> MFLYNLTLQRATGISFAIHGNFSGTKQQEIVVSRGKILELLRPDPNTGKVHTLLTVEVFGVIRSLMAFRLTGGTKDYIVVGSDSGRIVILEYQPSKNMFEKIHQETFGKSGCRRIVPGQFLAVDPKGRAVMISAIEKQKLVYILNRDAAARLTISSPLEAHKANTLVYHVVGVDVGFENPMFACLEMDYEEADNDPTGEAAANTQQTLTFYELDLGLNHVVRKYSEPLEEHGNFLITVPGGSDGPSGVLICSENYITYKNFGDQPDIRCPIPRRRNDLDDPERGMIFVCSATHKTKSMFFFLAQTEQGDIFKITLETDEDMVTEIRLKYFDTVPVAAAMCVLKTGFLFVASEFGNHYLYQIAHLGDDDEEPEFSSAMPLEEGDTFFFQPRPLKNLVLVDELDSLSPILFCQIADLANEDTPQLYVACGRGPRSSLRVLRHGLEVSEMAVSELPGNPNAVWTVRRHIEDEFDAYIIVSFVNATLVLSIGETVEEVTDSGFLGTTPTLSCSLLGDDALVQVYPDGIRHIRADKRVNEWKTPGKKTIVKCAVNQRQVVIALTGGELVYFEMDPSGQLNEYTERKEMSADVVCMSLANVPPGEQRSRFLAVGLVDNTVRIISLDPSDCLQPLSMQALPAQPESLCIVEMGGTEKQDELGERGSIGFLYLNIGLQNGVLLRTVLDPVTGDLSDTRTRYLGSRPVKLFRVRMQGQEAVLAMSSRSWLSYSYQSRFHLTPLSYETLEFASGFASEQCPEGIVAISTNTLRILALEKLGAVFNQVAFPLQYTPRKFVIHPESNNLIIIETDHNAYTEATKAQRKQQMAEEMVEAAGEDERELAAEMAAAFLNENLPESIFGAPKAGNGQWASVIRVMNPIQGNTLDLVQLEQNEAAFSVAVCRFSNTGEDWYVLVGVAKDLILNPRSVAGGFVYTYKLVNNGEKLEFLHK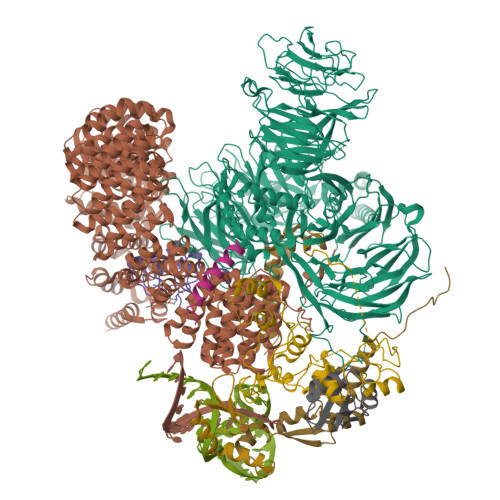TPVEEVPAAIAPFQGRVLIGVGKLLRVYDLGKKKLLRKCENKHIANYISGIQTIGHRVIVSDVQESFIWVRYKRNENQLIIFADDTYPRWVTTASLLDYDTVAGADKFGNICVVRLPPNTNDEVDEDPTGNKALWDRGLLNGASQKAEVIMNYHVGETVLSLQKTTLIPGGSESLVYTTLSGGIGILVPFTSHEDHDFFQHVEMHLRSEHPPLCGRDHLSFRSYYFPVKNVIDGDLCEQFNSMEPNKQKNVSEELDRTPPEVSKKLEDIRTRYAF;> MTDRYTIHSQLEHLQSKYIGTGHADTTKWEWLVNQHRDSYCSYMGHFDLLNYFAIAENESKARVRFNLMEKMLQPCGPPADKPEEN;> MAKIAKTHEDIEAQIREIQGKKAALDEAQGVGLDSTGYYDQEIYGGSDSRFAGYVTSIAATELEDDDDDYSSSTSLLGQKKPGYHAPVALLNDIPQSTEQYDPFAEHRPPKIADREDEYKKHRRTMIISPERLDPFADGGKTPDPKMNARTYMDVMREQHLTKEEREIRQQLAEKAKAGELKVVNGAAASQPPSKRKRRWDQTADQTPGATPKKLSSWDQAETPGHTPSLRWDETPGRAKGSETPGATPGSKIWDPTPSHTPAGAATPGRGDTPGHATPGHGGATSSARKNRWDETPKTERDTPGHGSGWAETPRTDRGGDSIGETPTPGASKRKSRWDETPASQMGGSTPVLTPGKTPIGTPAMNMATPTPGHIMSMTPEQLQAWRWEREIDERNRPLSDEELDAMFPEGYKVLPPPAGYVPIRTPARKLTATPTPLGGMTGFHMQTEDRTMKSVNDQPSGNLPFLKPDDIQYFDKLLVDVDESTLSPEEQKERKIMKLLLKIKNGTPPMRKAALRQITDKAREFGAGPLFNQILPLLMSPTLEDQERHLLVKVIDRILYKLDDLVRPYVHKILVVIEPLLIDEDYYARVEGREIISNLAKAAGLATMISTMRPDIDNMDEYVRNTTARAFAVVASALGIPSLLPFLKAVCKSKKSWQARHTGIKIVQQIAILMGCAILPHLRSLVEIIEHGLVDEQQKVRTISALAIAALAEAATPYGIESFDSVLKPLWKGIRQHRGKGLAAFLKAIGYLIPLMDAEYANYYTREVMLILIREFQSPDEEMKKIVLKVVKQCCGTDGVEANYIKTEILPPFFKHFWQHRMALDRRNYRQLVDTTVELANKVGAAEIISRIVDDLKDEAEQYRKMVMETIEKIMGNLGAADIDHKLEEQLIDGILYAFQEQTTEDSVMLNGFGTVVNALGKRVKPYLPQICGTVLWRLNNKSAKVRQQAADLISRTAVVMKTCQEEKLMGHLGVVLYEYLGEEYPEVLGSILGALKAIVNVIGMHKMTPPIKDLLPRLTPILKNRHEKVQENCIDLVGRIADRGAEYVSAREWMRICFELLELLKAHKKAIRRATVNTFGYIAKAIGPHDVLATLLNNLKVQERQNRVCTTVAIAIVAETCSPFTVLPALMNEYRVPELNVQNGVLKSLSFLFEYIGEMGKDYIYAVTPLLEDALMDRDLVHRQTASAVVQHMSLGVYGFGCEDSLNHLLNYVWPNVFETSPHVIQAVMGALEGLRVAIGPCRMLQYCLQGLFHPARKVRDVYWKIYNSIYIGSQDALIAHYPRIYNDDKNTYIRYELDYIL;> MAKHHPDLIFCRKQAGVAIGRLCEKCDGKCVICDSYVRPCTLVRICDECNYGSYQGRCVICGGPGVSDAYYCKECTIQEKDRDGCPKIVNLGSSKTDLFYERKKYGFKKR;> AAAAARAARAAAWRAEQAAAA;> MATEHPEPPKAELQLPPPPPPGHYGAWAAQELQAKLAEIGAPIQGNREELVERLQSYTRQTGIVLNRPVLRGEDGDKAAPPPMSAQLPGIPMPPPPLGLPPLQPPPPPPPPPPGLGLGFPMAHPPNLGPPPPLRVGEPVALSEEERLKLAQQQAALLMQQEERAKQQGDHSLKEHELLEQQKRAAVLLEQERQQEIAKMGTPVPRPPQDMGQIGVRTPLGPRVAAPVGPVGPTPTVLPMGAPVPRPRGPPPPPGDENREMDDPSVGPKIPQALEKILQLKESRQEEMNSQQEEEEMETDARSSLGQSASETEEDTVSVSKKEKNRKRRNRKKKKKPQRVRGVSSESSGDREKDSTRSRGSDSPAADVEIEYVTEEPEIYEPNFIFFKRIFEAFKLTDDVKKEKEKEPEKLDKLENSAAPKKKGFEEEHKDSDDDSSDDEQEKKPEAPKLSKKKLRRMNRFTVAELKQLVARPDVVEMHDVTAQDPKLLVHLKATRNSVPVPRHWCFKRKYLQGKRGIEKPPFELPDFIKRTGIQEMREALQEKEEQKTMKSKMREKVRPKMGKIDIDYQKLHDAFFKWQTKPKLTIHGDLYYEGKEFETRLKEKKPGDLSDELRISLGMPVGPNAHKVPPPWLIAMQRYGPPPSYPNLKIPGLNSPIPESCSFGYHAGGWGKPPVDETGKPLYGDVFGTNAAEFQTKTEEEEIDRTPWGELEPSDEESSEEEEEEESDEDKPDETGFITPADSGLITPGGFSSVPAGMETPELIELRKKKIEEAMDGSETPQLFTVLPEKRTATVGGAMMGSTHIYDMSTVMSRKGPAPELQGVEVALAPEELELDPMAMTQKYEEHVREQQAQVEKEDFSDMVAEHAAKQKQKKRKAQPQDSRGGSKKYKEFKF;> MAAGPISERNQDATVYVGGLDEKVSEPLLWELFLQAGPVVNTHMPKDRVTGQHQGYGFVEFLSEEDADYAIKIMNMIKLYGKPIRVNKASAHNKNLDVGANIFIGNLDPEIDEKLLYDTFSAFGVILQTPKIMRDPDTGNSKGYAFINFASFDASDAAIEAMNGQYLCNRPITVSYAFKKDSKGERHGSAAERLLAAQNPLSQADRPHQLFADAPPPPSAPNPVVSSLGSGLPPPGMPPPGSFPPPVPPPGALPPGIPPAMPPPPMPPGAAGHGPPSAGTPGAGHPGHGHSHPHPFPPGGMPHPGMSQMQLAHHGPHGLGHPHAGPPGSGGQPPPRPPPGMPHPGPPPMGMPPRGPPFGSPMGHPGPMPPHGMRGPPPLMPPHGYTGPPRPPPYGYQRGPLPPPRPTPRPPVPPRGPLRGPLPQ;> MDFQHRPGGKTGSGGVASSSESNRDRRERLRQLALETIDINKDPYFMKNHLGSYECKLCLTLHNNEGSYLAHTQGKKHQTNLARRAAKEAKEAPAQPAPEKVKVEVKKFVKIGRPGYKVTKQRDSEMGQQSLLFQIDYPEIAEGIMPRHRFMSAYEQRIEPPDRRWQYLLMAAEPYETIAFKVPSREIDKAEGKFWTHWNRETKQFFLQFHFKMEKPPAPPSLPAGPPGVKRPPPPLMNGLPPRPPLPESLPPPPPGGLPLPPMPPTGPAPSGPPGPPQLPPPAPGVHPPAPVVHPPASGVHPPAPGVHPPAPGVHPPAPGVHPPTSGVHPPAPGVHPPAPGVHPPAPGVHPPAPGVHPPAPGVHPPPSAGVHPQAPGVHPAAPAVHPQAPGVHPPAPGMHPQAPGVHPQPPGVHPSAPGVHPQPPGVHPSNPGVHPPTPMPPMLRPPLPSEGPGNIPPPPPTN;> METILEQQRRYHEEKERLMDVMAKEMLTKKSTLRDQINSDHRTRAMQDRYMEVSGNLRDLYDDKDGLRKEELNAISGPNEFAEFYNRLKQIKEFHRKHPNEICVPMSVEFEELLKARENPSEEAQNLVEFTDEEGYGRYLDLHDCYLKYINLKASEKLDYITYLSIFDQLFDIPKERKNAEYKRYLEMLLEYLQDYTDRVKPLQDQNELFGKIQAEFEKKWENGTFPGWPKETSSALTHAGAHLDLSAFSSWEELASLGLDRLKSALLALGLKCGGTLEERAQRLFSTKGKSLESLDTSLFAKNPKSKGTKRDTERNKDIAFLEAQIYEYVEILGEQRHLTHENVQRKQARTGEEREEEEEEQISESESEDEENEIIYNPKNLPLGWDGKPIPYWLYKLHGLNINYNCEICGNYTYRGPKAFQRHFAEWRHAHGMRCLGIPNTAHFANVTQIEDAVSLWAKLKLQKASERWQPDTEEEYEDSSGNVVNKKTYEDLKRQGLL> MKITVRGSEMVYPAAETPRRRLWNSGPDLVVPRFHTPSVYFFRRRDADGNDLTAADGSFFDGARMRRALAEALVPFYPMAGRLARDE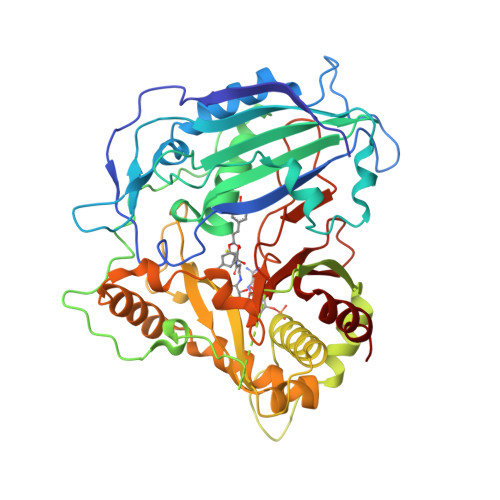DGRVEIDCNAAGVLFQEADAPDATIDYFGDFAPTMELKRLIPTVDFSDDTAFPLLVLQVTHFKCGGVAIGVGMQHHVADGFSGLHFINSWADLCRGVPIAVMPFIDRSLLRARDPPAPVYPHVEYQPAPAMLSSEPPQAALTAKPATPPAAVAIFKLSRAELGRLRSQVPAREREGAPRFSTYAVLAAHVWRCASLARGLPADQPTKLYCATDGRQRLQPPLPEGYFGNVIFTATPLANAGTVTAGVAEGAAVIQAALDRMDDGYCRSALDYLELQPDLSALVRGAHTFRCPNLGLTSWVRLPIHDADFGWGRPVFMGPGGIAYEGLAFVLPSANRDGSLSVAISLQAEHMEKFRKLIYDF>[2x]GCGGKKGSSDNTSTLAMIDSVDAHGLQRMQTSKSETDFKFKGKDYHSLVSRTPDDNLPHVTNELGDTYVDNKIVLHLTRGNETVLNKTFTKNDFSSVVD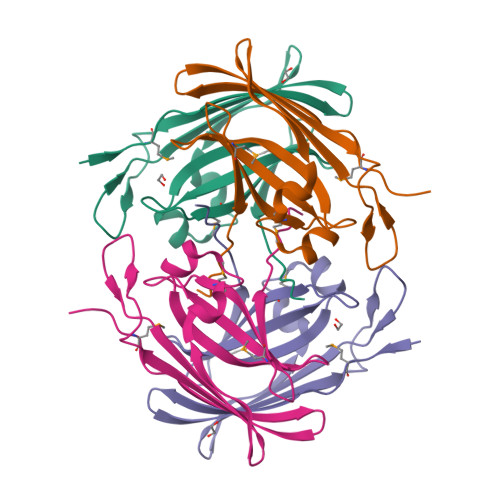ANFLSKSILEGIVYDKTTPQGIVYAASVCYPQTDLYMPLSITITADGKMSIQKVDILEEDYDDEAPN> SNAMTALKVGSESWWQSKHGPEWQRLNDEMFEVTFWWRDPQGSEEYSTIKRVWVYITGVTDHHQNSQPQSMQRIAGTDVWQWTTQLNANWRGSYCFIPTERDDIFSAPSPDRLELREGWRKLLPQAIADPLNPQSWKGGLGHAVSALEMPQAPLQPGWDCPQAPEIPAKEIIWKSERLKNSRRVWIFTTGDVTAEERPLA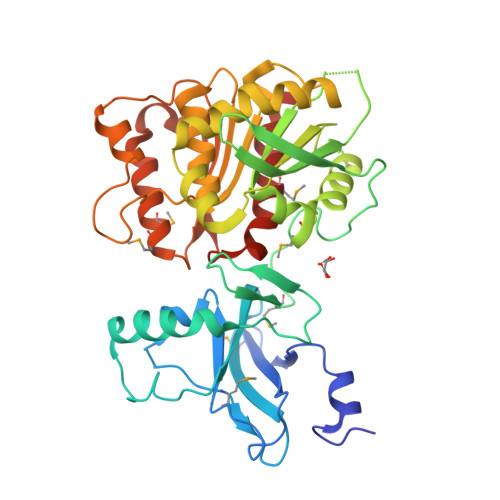VLLDGEFWAQSMPVWPVLTSLTHRQQLPPAVYVLIDAIDTTHRAHELPCNADFWLAVQQELLPLVKVIAPFSDRADRTVVAGQSFGGLSALYAGLHWPERFGCVLSQSGSYWWPHRGGQQEGVLLEKLKAGEVSAEGLRIVLEAGIREPMIMRANQALYAQLHPIKESIFWRQVDGGHDALCWRGGLMQGLIDLWQPLFHDRS>[4x]MSQSQRSTADWQRLDAAHHLHPFTDYGELNTKGSRIITRAEGCYLWDSDGNQILDGMAGLWCVNIGYGRKELAEVAYRQMQELPYYNNFFQCSHPPAIELSRLLSEVTPKHMNHVFFTGSGSDSNDTILRMVRYYWKLLGKPYKKVVISRENAYHGSTVAGASLSGMKAMHSHGDLPIPGIEHIEQPYHFGRAPDMDPAEFGRQAAQALERKIDEIGECNVAAFIAEPIQGAGGVIIPP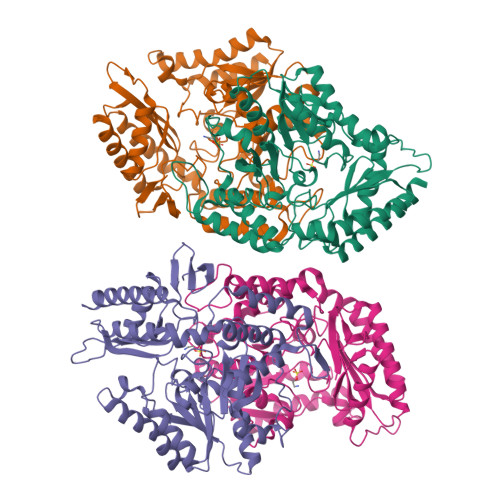DSYWPEIKRICAERDILLIVDEVITGFGRLGTWFGSQYYDLQPDLMPIAKGLSSGYMPIGGVMVSDRVAKVVIEEGGEFFHGYTYSGHPVAAAVAAENIRIMRDEGIIERAGAEIAPYLQARWRELGEHPLVGEARGVGMVAALELVKSKQPLERFEEPGKVGSLCRDLSVKNGLVMRAVGGTMIISPPLVLSREQVDELIDKARRTLDETHKAIGGALEHHHHHH Examples include herpesviruses and most bacteriophages, both of which replicate their DNA as head-to-tail concatemers containing multiple copies of the genome that must be cleaved to generate unit-length viral genomes. This is achieved using a “terminase” complex, which, in bacteriophages comprises two proteins, termed Large (TerL) and Small (TerS) terminases; but in herpesviruses contains three separate components—pUL15, pUL28 and pUL33—in hitherto unknown oligomeric forms. The terminase complex recognizes a specific sequence or structure on the concatemeric DNA and cuts it to produce the free end where packaging is initiated. Acting as the packaging motor, the terminase complex then hydrolyzes ATP molecules to translocate negatively charged DNA into a space-limited procapsid through a dodecameric portal (Chen, 2020; Nan Wang, et al. 2020). Each subunit of the hexameric ring is a heterotrimer formed by three proteins (pUL15, pUL28 and pUL33) interdigitating with each other.

By using the block-reconstruction method, we were able to improve the resolution for the structures of the hexameric and dodecameric terminases to 3.5 Å and 3.6 Å, respectively, suggesting that the complex is intrinsically flexible with unrestrained symmetry. The backbone of the polypeptide, as well as most side chains, were clearly defined, allowing an atomic model of the terminase complex to be built de novo. The 85-kDa pUL28 (which has no sequence or predicted structural similarities with bacteriophage TerS) and 15-kDa pUL33 remain enigmatic for their structures and functions. pUL28 folds into six distinct domains: spool (residues 1–119), fix (residues 120–191 and 533–563), strut (residues 192–226), reinforce (residues 227–413 and 510–532), regulator (residues 414–509) and packing (residues 564–775) based on its roles in initializing the assembly of the terminase complex, and all domains are engaged in extensive associations with pUL15 (interaction area ~6,700 Å2). pUL33, consisting primarily of five helices, threads through a compact “triangle” formed by the spool, fix, strut and reinforce domains of pUL28, thus firmLy stabilized by extensive interactions with pUL28 (contact area ~4,500 Å2). In turn, the pUL28 N-terminal spool domain is twined around by two N-lasso domains of pUL15 and pUL33, further facilitating the assembly of the complex. Unexpectedly, our structure reveals an intermolecular Zn finger formed by residues C121 and H124 from pUL28 fix domain, and residues C101 and H103 from pUL33, which are highly conserved across the herpesvirus family. Furthermore, the pUL28 fix domain, comprising a three-helix-bundle plus an antiparallel two-stranded β-sheet, appears to fix the orientation of the pUL33 C-domain. Two clusters of three-helix bundles formed by the strut domains of pUL15 and pUL28 support each other, along with a second intramolecular Zn finger (residues C197, C200, C223 and H225 from pUL28), immobilizing the “backbone” of the ATPase domain.

> TMGGDALRVPFLDFATATPKRHQTVVPGVGTLHDCCEHSPLFSAVARRLLFNSLVPAQLKGRDFGGDHTAKLEFLAPELVRAVARLRFKECAPADVVPQRNAYYSVLNTFQALHRSEAFRQLVHFVRDFAQLLKTSFRASSLTETTGPPKKRAKVDVATHGRTYGTLELFQKMILMHATYFLAAVLLGDHAEQVNTFLRLVFEIPLFSDAAVRHFRQRATVFLVPRRHGKTWFLVPLIALSLASFRGIKIGYTAHIRKATEPVFEEIDACLRGWFGSARVDHVKGETISFSFPDGSRSTIVFASSHNTNGIRGQDFNLLFVDEANFIRPDAVQTIMGFLNQANCKIIFVSSTNTGKASTSFLYNLRGAADELLNVVTYICDDHMPRVVTHTNATACSCYILNKPVFITMDGAVRRTADLFLADSFMQEIIGGQARETGDDRPVLTKSAGERFLLYRPSTTTNSGLMAPDLYVYVDPAFTANTRASGTGVAVVGRYRDDYIIFALEHFFLRALTGSAPADIARCVVHSLTQVLALHPGAFRGVRVAVEGNSSQDSAVAIATHVHTEMHRLLASEGADAGSGPELLFYHCEPPGSAVLYPFFLLNKQKTPAFEHFIKKFNSGGVMASQEIVSATVRLQTDPVEYLLEQLNNLTETVSPNTDVRTYSGKRNGASDDLMVAVIMAIYLAAQAGPPHTF;> AAPVSEPTVARQKLLALLGQVQTYVFQIELLRRCDPHIGRGKLPQLKLNALQVRALRRRLRPGLEAQAGAFLTPLSVTLELLLEYAWREGERLLGSLETFATAGDVAAFFTETMGLARPCPYHQRVRLDTYGGTVHMELCFLHDVENFLKQLNYCHLITPSRGATAALERVREFMVGAVGSGLIVPPELSDPSHPCAVCFEELCVTANQGATIASRLADRICNHVTQQAQVRLDANELRRYLPHAAGLSDADRARALSVLDHALARTAGGDGQPHPSPENDSVRKEADALLEAHDVFQATTPGLYAISELQFWLASGDRAGQTTMDAFASNLTALARRELQQETAAVAVELALFGRRAEHFDRAFGSHLAALDMVDALIIGGQATSPDDQIEALIRACYDHHLTTPLLRRLVSPEQCDEEALRRVLARMGAGGAADAPKGGAGPDDDGDRVAVEEGARGLGAPGGGGEDEDRRRGPGGQGPETWGDIATQAAADVRERRRLYADRLTKRSLASLGRCVREQRGELEKMLRVSVHGEVLPATFAAVANGFAARARFCALTAGAGTVIDNRSAPGVFDAHRFMRASLLRHQVDPALLPSITHRFFELVNGPLFDHSTHSFAQPPNTALYYSVENVGLLPHLKEELARFIMGAGGSGADWAVSEFQRFYCFDGISGITPTQRAAWRYIRELIIATTLFASVYRCGELELRRPDCSRPTSEGRYRYPPGVYLTYDSDCPLVAIVESAPDGCIGPRSVVVYDRDVFSILYSVLQHLAPR;> TLRDTIPDCALRSQTLESLDARYVSRDGAHDAAVWFEDMTPAELEVVFPTTDAKLNYLSRTQRLASLLTYAGPIKAPDDAAAPQTPDTACVHGELLARKRERFAAVINRFLDLHQILR>HMERDEVGAHKNAVDEEIERLSQPGGSEDQRLNALAERFGGVLLSEIYDDVSLEDAPYFSALYGPSRHAIVVPDLSQVTEHLEGLTDCPEDLYLIEGDPQSFDDSVFSVDELEKAVVVKIADRQWRYSRFPEV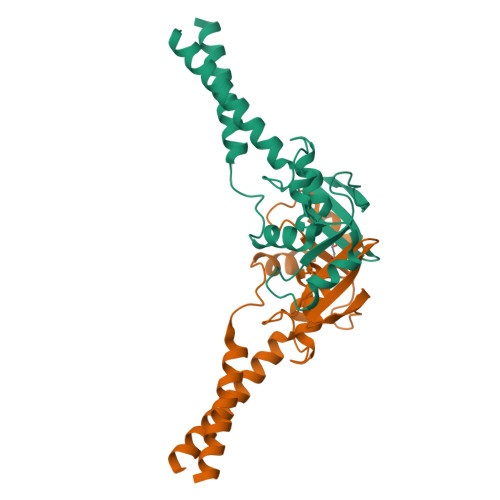PLFGRAARESRIESLHAEREVLSERFATL[2x]Intracellular replication of L. pneumophila requires functional Dot/Icm T4BSS, irrespectively of host species. It has been well established that L. pneumophila translocate more than 100 effector proteins into host cytoplasm using the Dot/Icm T4BSS. The complex is supposed to contain two outer membrane lipoproteins, DotC and DotD, two inner membrane-spanning proteins, DotF and DotG, and one outer membrane-associated protein, DotH. The outer membrane targeting of DotH depends on lipoproteins DotC and DotD, presumably in a manner analogous with the function of pilotin in targeting secretin inT2SS: the outer membrane lipoprotein pilotin is required for the stabilization and outer membrane targeting of the secretin. In conclusion, the present study revealed that the structurally conserved DotD/N0/T3S domain is widely spread throughout outer membrane complexes of even distantly related secretion systems, including T2SS, T3SS and T4BSS.

To clarify the structure and the molecular mechanism of Dot/Icm T4BSS, we crystallized DotD without the first 20 amino acids which contain the signal sequence for secretion across inner membranes and the lipidation site, Cys20 (DotDΔN), and determined the structure at 2.0 Å resolution. DotDΔN is composed of the compact C-terminal domain (DotD domain) and the N-terminal disordered region. The N-terminal third of DotDΔN was invisible in the electron density map, except for a short β-strand (Ala-37 to Ala-42) that we call the “lid. The DotD domain forms a βαβ sandwich fold composed of two α-helices flanked by an antiparallel three-stranded β-sheet on one side and a mixed three-stranded β-sheet on the other side. DaliLite database search showed that the DotD domain has striking structural similarity to the N-terminal subdomain of secretins, which are outer membrane pore-forming proteins of T2SS and T3SS. Thus the DotD domain and the N0/T3S domains of the type II/III secretins share remarkable structural homology, although they are poorly related in amino acid sequences. The most remarkable difference between DotD and the N0/T3S domains of secretins is that DotD has a lid that makes β-strand addition to β-strands β1 and β3. The lid is located on β1 and covers the hydrophobic cleft formed by α1, α2 and β1. The side chains of two hydrophobic residues in the lid (Ile-39 and Leu-41) stick into the cleft.

> GSHMAGTMKFKKPPINNPSDDATIKLAEAAVSVSDSMLEMAKVEKVITPPSKDNTLTIPNAYNLQARASVDWSGPIEELTARIAKAAHFRFRVLGKSPSVPVLISISTKDESLAEILRDIDYQAGKKASIHVYPNSQVVELRYAKIYS>MEQPGLCGLSNLGNTCFMNSAIQCLSNTPPLTEYFLNDKYQEELNFDNPLGMRGEIAKSYAELIKQMWSGKFSYVTPRAFKTQVGRFAPQFSGYQQQDCQELLAFLLDGLHEDLNRIRKKPYIQLKDADGRPDKVVAEEAWENHLKRNDSIIVDIFHGLFKSTLVCPECAKISVTFDPFCYLTLPLASTSKVKLKDCIELFTTKEKLGAEDPWYCPNCKEHQQATKKLDLWSLPPVLVVHLKRFSYSRYMRDKLDTLVDFPINDLDMSEFLINPNAGPCRYNLIAVSNHYGGMGGGHYTAFAKNKDDGKWYYFDDSSV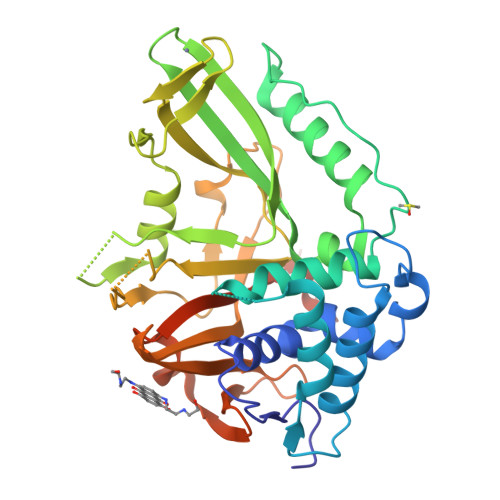STASEDQIVSKAAYVLFYQRQDTFSGTGFFPLDRETAAALEHHHHHH[2x]> 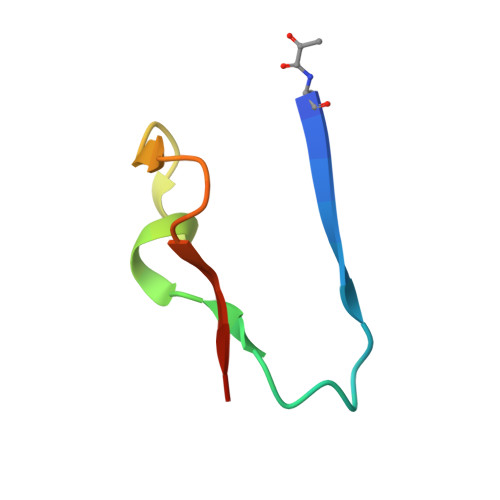XSFALGLRKDCRAEIVEKFTEPGTVIRINEVVAALKA> MGEQPIFSTRAHVFQIDPNTKKNWVPTSKHAVTVSYFYDSTRNVYRIISLDGSKAIINSTITPNMTFTKTSQKFGQWADSRANTVYGLGFSSEHHLS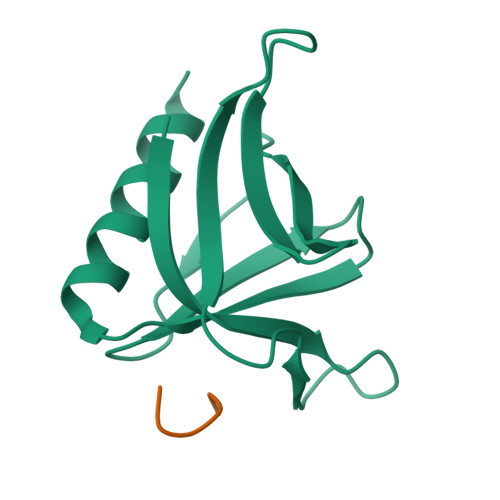KFAEKFQEFKEAAR;> TPPSPF3',3'-cdIMP | C20 H22 N8 O14 P2 | 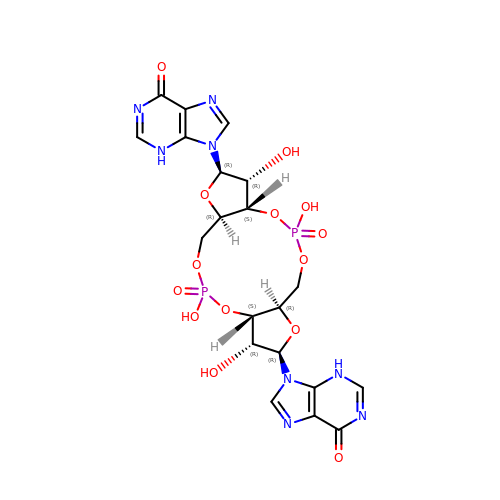VFTRASQVWRBMKD-XPWFQUROSA-N> YDPTKAGDIVKATKWPPKLPEIQDLAIRARVFIHKSTIKD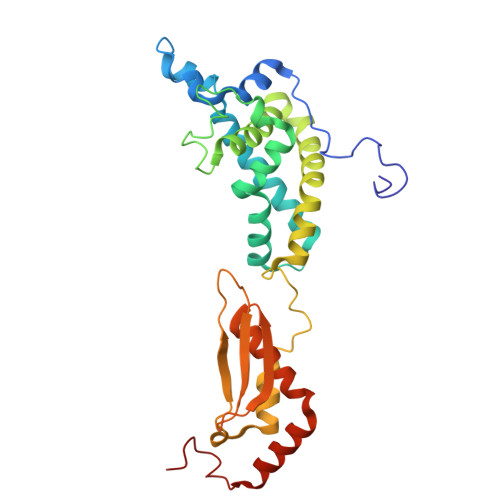KVYLSGSEMINAHNERLEFLGDSILNSVMTLIIYNKFPDYSEGQLSTLRMNLVSNEQIKQWSIMYNFHEKLKTNFDLKDENSNFQNGKLKLYADVFEAYIGGLMEDDPRNNLPKIRKWLRKLAKPVIEEATRNQVALEKTDKLDMNAKRQLYSLIGYASLRLHYVTVKKPTAVDPNSIVECRVGDGTVLGTGVGRNIKIAGIRAAENALRDKKMLDFYAKQRAAIPRSESVLKDPS> GGPGPRVVVIGAGLAGLAAAKALLEQGFTDVTVLEASSHIGGRVQSVKLGHATFELGATWIHGSHGNPIYHLAEANGLLEETTDGERSVGRISLYSKNGVACYLTNHGRRIPKDVVEEFSDLYNEVYNLTQEFFRHDKPVNAESQNSVGVFTREEVRNRIRNDPDDPEATKRLKLAMIQQYLKVESCESSSHSMDEVSLSAF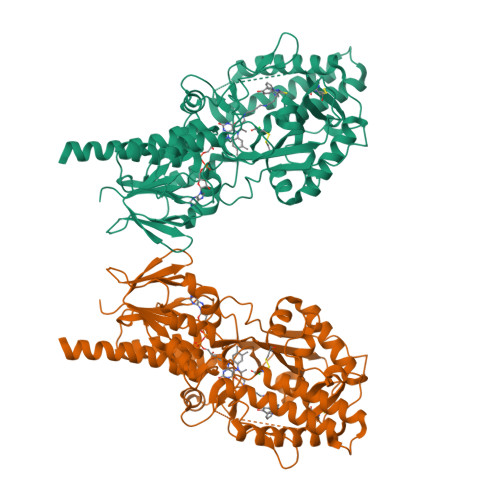GEWTEIPGAHHIIPSGFMRVVELLAEGIPAHVIQLGKPVRCIHWDQASGSGSGSVVVECEDCELIPADHVIVTVSLGVLKRQYTSFFRPGLPTEKVAAIHRLGIGTTDKIFLEFEEPFWGPECNSLQFVWEDEAESHTLTYPPELWYRKICGFDVLYPPERYGHVLSGWICGEEALVMETLSDEAVAEICTEMLRQFTGNPNIPKPRRILRSAWGSNPYFRGSYSYTQVGSSGADVEKLAKPLPGLQVLFSGEATHRKYYSTTHGALLSGQREAARLIEMYRDLFQQSRPRL>MQMMTRKVLLNMELEEDDDEDGDIVLENFDQTIVCPTFGSLENQQDFRTPEFEEFNGKPDSLFFTDGQRRIDFILVYEDESKKENNKKGTNEKQKRKRQAYESNLICHGLQLEATRSVSDDKLVFVKVHAPWEVLCTYAEIMHIKLPLKPNDLKTRSPFGNLNWFTKVLRVNESVIKPEQEFFTAPFEKSRMNDFYILDRDSFFNPATRSRIVYFILSRVKYQVMNNVNKFGINRLVSSGIYKAAFPLHDCRFNYESEDISCPSERYLLYREWAHPRSIYKKQPLDLIRKYYGEKIGIYFAWLGYYTQMLLLAAVVGVACFLYGYLDQDNCTWSKEVCDPDIGGQILMCPQCDRLCPFWRLNITCESSKKLCIFDSFGTLIFAVFMGVWVTLFLEFWKRRQAELEYEWDTVELQQEEQARPEYEAQCNHVVINEITQEEERIPFTTCGKCIRVTLCASAVFFWILLIIASVIGIIVYRLSVFIVFSTTLPKNPNGTDPIQKYLTPQMATSITASIISFIIIMILNTIYEKVAIMITNFELPRTQTDYENSLTMKMFLFQFVNYYSSCFYIAFFKGKFVGYPGDPVYLLGKYRSEECDPGGCLLELTTQLTIIMGGKAIWNNIQEVLLPWVMNLIGRYKRVSGSEKITPRWEQDYHLQPMGKLGLFYEYLEMIIQFGFVTLFVASFPLAPLLALVNNILEIRVDAWKLTTQFRRMVPEKAQDIGAWQPIMQGIAILAVVTNAMIIAFTSDMIPRLVYYWSFSIPPYGDHTYYTMD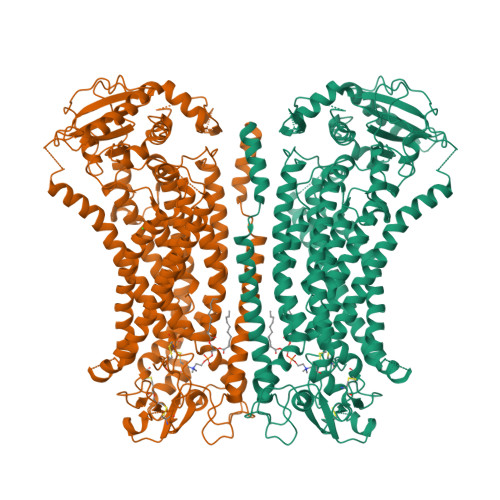GYINNTLSVFNITDFKNTDKENPYIGLGNYTLCRYRDFRNPPGHPQEYKHNIYYWHVIAAKLAFIIVMEHIIYSVKFFISYAIPDVSKITKSKIKREKYLTQKLLHESHLKDLTKNMGIIAERIGGTVDNSVRPKLE[2x]> DYIPEPMDLSLVDLPESLIQLSERIAENVHEVWAKARIDEGWTYGEKRDDIHKKHPCLVPYDELPEEEKEYDRNTAMNTIKMVKKLGFRIEKEDEKAEDNLKKTKLPKTYMMSNMKENKLDYIPEPMDLSLVDLPESLIQLSERIAENVHEVWAKARIDEGWTYGEKRDDI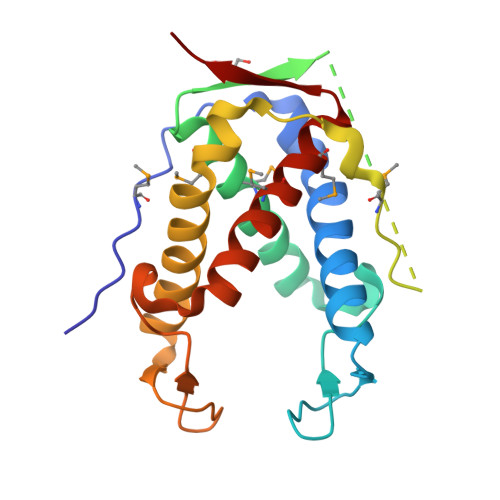HKKHPCLVPYDELPEEEKEYDRNTAMNTIKMVKKLGFRIEKED Transcription initiation in bacteria involves the recruitment of RNAP by sigma factors (σ) to promoter regions located upstream from the transcription start site (TSS, position +1). In approximately 60% of bacteria, a major variant σ factor, σ54, forms a class of its own, lacking structural and sequence similarity to σ70. In σ54-mediated transcription initiation, σ54 recruits RNAP to genes responsible for regulating a variety of stress responses, including nutrient depletion, membrane stress, antibiotic exposure, and biofilm formation. In this study, we used single-particle cryo-electron microscopy (cryoEM) to determine the structures of initial transcribing complexes of increasing RNA lengths from 5 nt to 9 nt, which allow us to propose a mechanism of RNAP promoter escape in the σ54 system.

In 8 and 9 nt complexes, the density for the RII-finger is partially lost, indicating this region becoming dynamic in nature and the interactions observed in 7 nt are lost. In addition, P110 and Y112, observed in 5 to 7nt complexes, were also not resolved, indicating that these interactions are no longer stably maintained. Further RNA extension releases RII-finger by breaking the hydrophobic interactions between the β′ lid and RII residues P110 and Y112. At RPitc-8nt and -9nt, both template and nontemplate strands scrunch around the ELH, losing interactions between the DNA strands and ELH, resulting in reduced density for both DNA and the ELH. Furthermore, we also observe the loss of resolution of the upstream DNA and upstream DNA binding domains on σ54 (RpoN, ELH-HTH), suggesting that both the σ54 upstream DNA binding subdomains and upstream DNA are less stably engaged with RNAP. Interestingly, the proportion of σ54-free complexes increases with increasing RNA lengths, suggesting that the σ54-RNAP complexes become increasingly unstable.

>[2x]SVTEFLKPRLVDIEQVSSTHAKVTLEPLERGFGHTLGNALRRILLSSMPGCAVTEVEIDGVLHEYSTKEGVQEDILEILLNLKGLAVRVQGKDEVILTLNKSGIGPVTAADITHDGDVEIVKPQHVICHLTDENASISMRIKVQRGRGYVPASTRIHSEEDERPIGRLLVDACYSPVERIAYNVEAARVEQRTDLDKLVIEMETNGTIDPEEAIRRAATILAEQLEAFVDLRDVRQPEVKEEKPEFDPILLRPVDDLELTVRSANCLKAEAIHYIGDLVQRTEVELLKTPNLGKKSLTEIKDVLASRGLSLGMRLENWPPA;> MVYSYTEKKRIRKDFGKRPQVLDVPYLLSIQLDSFQKFIEQDPEGQYGLEAAFRSVFPIQSYSGNSELQYVSYRLGEPVFDVQECQIRGVTYSAPLRVKLRLVIYEREAPEGTVKDIKEQEVYMGEIPLMTDNGTFVINGTERVIVSQLHRSPGVFFDSDKGKTHSSGKVLYNARIIPYRGSWLDFEFDPKDNLFVRIDRRRKLPATIILRALNYTTEQILDLFFEKVIFEIRDNKLQMELVPERLRGETASFDIEANGKVYVEKGRRITARHIRQLEKDDVKLIEVPVEYIAGKVVAKDYIDESTGELICAANMELSLDLLAKLSQSGHKRIETLFTNDLDHGPYISETLRVDPTNDRLSALVEIYRMMRPGEPPTREAAESLFENLFFSEDRYDLSAVGRMKFNRSLLREEIEGSGILSKDDIIDVMKKLIDIRNGKGEVDDIDHLGNRRIRSVGEMAENQFRVGLVRVERAVKERLSLGDLDTLMPQDMINAKPISAAVKEFFGSSQLSQFMDQNNPLSEITHKRRISALGPGGLTRERAGFEVRDVHPTHYGRVCPIETPEGPNIGLINSLSVYAQTNEYGFLETPYRKVTDGVVTDEIHYLSAIEEGNYVIAQANSNLDEEGHFVEDLVTCRSKGESSLFSRDQVDYMDVSTQQVVSVGASLIPFLEHDDANRALMGANMQRQAVPTLRADKPLVGTGMERAVAVDSGVTAVAKRGGVVQYVDASRIVIKVNEDEMYPGEAGIDIYNLTKYTRSNQNTCINQMPCVSLGEPVERGDVLADGPSTDLGELALGQNMRVAFMPWNGYNFEDSILVSERVVQEDRFTTIHIQELACVSRDTKLGPEEITADIPNVGEAALSKLDESGIVYIGAEVTGGDILVGKVTPKGETQLTPEEKLLRAIFGEKASDVKDSSLRVPNGVSGTVIDVQVFTRDGVEKDKRALEIEEMQLKQAKKDLSEELQILEAGLFSRIRAVLVAGGVEAEKLDKLPRDRWLELGLTDEEKQNQLEQLAEQYDELKHEFEKKLEAKRRKITQGDDLAPGVLKIVKVYLAVKRRIQPGDKMAGRHGNKGVISKINPIEDMPYDENGTPVDIVLNPLGVPSRMNIGQILETHLGMAAKGIGDKINAMLKQQQEVAKLREFIQRAYDLGADVRQKVDLSTFSDEEVMRLAENLRKGMPIATPVFDGAKEAEIKELLKLGDLPTSGQIRLYDGRTGEQFERPVTVGYMYMLKLNHLVDDKMHARSTGSYSLVTQQPLGGKAQFGGQRFGEMEVWALEAYGAAYTLQEMLTVKSDDVNGRTKMYKNIVDGNHQMEPGMPESFNVLLKEIRSLGINIELED;> LLKFLKAQTKTEEFDAIKIALASPDMIRSWSFGEVKKPETINYRTFKPERDGLFCARIFGPVKDYECLCGKYKRLKHRGVICEKCGVEVTQTKVRRERMGHIELASPTAHIWFLKSLPSRIGLLLDMPLRDIERVLYFESYVVIEGGMTNLERQQILTEEQYLDALEEFGDEFDAKMGAEAIQALLKSMDLEQECEQLREELNETNSETKRKKLTKRIKLLEAFVQSGNKPEWMILTVLPVLPPDLRPLVPLDGGRFATSDLNDLYRRVINRNNRLKRLLDLAAPDIIVRNEKRMLQEAVDALLDNGRRGRAITGSNKRPLKSLADMIKGKQGRFRQNLLGKRVDYSGRSVITVGPYLRLHQCGLPKKMALELFKPFIYGKLELRGLATTIKAAKKMVEREEAVVWDILDEVIREHPVLLNRAPTLHRLGIQAFEPVLIEGKAIQLHPLVCAAYNADFDGDQMAVHVPLTLEAQLEARALMMSTNNILSPANGEPIIVPSQDVVLGLYYMTRDCVNAKGEGMVLTGPKEAERLYRSGLASLHARVKVRITEYEKDANGELVAKTSLKDTTVGRAILWMIVPKGLPYSIVNQALGKKAISKMLNTCYRILGLKPTVIFADQIMYTGFAYAARSGASVGIDDMVIPEKKHEIISEAEAEVAEIQEQFQSGLVTAGERYNKVIDIWAAANDRVSKAMMDNLQTETVINRDGQEEKQVSFNSIYMMADSGARGSAAQIRQLAGMRGLMAKPDGSIIETPITANFREGLNVLQYFISTHGARKGLADTALKTANSGYLTRRLVDVAQDLVVTEDDCGTHEGIMMTPVIEGGDVKEPLRDRVLGRVTAEDVLKPGTADILVPRNTLLHEQWCDLLEENSVDAVKVRSVVSCDTDFGVCAHCYGRDLARGHIINKGEAIGVIAAQSIGEPGTQLTMRTFHIGGAASRAAAESSIQVKNKGSIKLSNVKSVVNSSGKLVITSRNTELKLIDEFGRTKESYKVPYGAVLAKGDGEQVAGGETVANWDPHTMPVITEVSGFVRFTDMIDGQTITRQTDELTGLSSLVVLDSAERTAGGKDLRPALKIVDAQGNDVLIPGTDMPAQYFLPGKAIVQLEDGVQISSGDTLARIPQESGGTKDITGGLPRVADLFEARRPKEPAILAEISGIVSFGKETKGKRRLVITPVDGSDPYEEMIPKWRQLNVFEGERVERGDVISDGPEAPHDILRLRGVHAVTRYIVNEVQDVYRLQGVKINDKHIEVIVRQMLRKATIVNAGSSDFLEGEQVEYSRVKIANRELEANGKVGATYSRDLLGITKASLATESFISAASFQETTRVLTEAAVAGKRDELRGLKENVIVGRLIPAGTGYAYHQDRMRRRAAG;> ARVTVQDAVEKIGNRFDLVLVAARRARQMQVGGKDPLVPEENDKTTVIALREIEEGLINNQILDVRERQEQQEQ;> GTPSGNGVDQGETTQSLQDYLMWQVELTPFTDTDRAIATSIVDAVDDTGYLTIQIEDIVDSIGDDEIGLEEVEAVLKRIQRFDPVGVAAKDLRDCLLIQLSQFAKETPWLEEARLIISDHLDLLANHDFRTLMRVTRLKEEVLKEAVNLIQSLDPRPGQSIQTGEPEYVIPDVLVRKVNDRWVVELNSSLESANDTLLRVSRCIVEQQQAFFEQGEEYMKPMVLADIAQAVEMHESTISRVTTQKYLHSPRGIFELKYFFSSHVNTEGGGEASSTAIRALVKKLIAAENPAKPLSDSKLTSMLSEQGIMVARRTVAKYRESLSIPPSNQ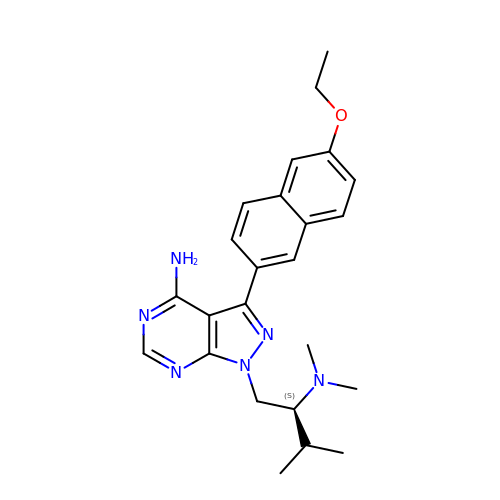1-[(2S)-2-(dimethylamino)-3-methylbutyl]-3-(6-ethoxynaphthalen-2-yl)-1H-pyrazolo[3,4-d]pyrimidin-4-amine | C24 H30 N6 O | UPGKXNICLSVZDA-HXUWFJFHSA-N β1,3-N-acetylglucosaminyltransferases (B3GNTs) are Golgi-resident glycosyltransferases involved in the biosynthesis of poly-N-acetyl-lactosamine chains. They catalyze the addition of the N-acetylglucosamine to the N-acetyl-lactosamine repeat as a key step of the chain elongation process. Among the characterized B3GNTs, B3GNT2 is the major poly-N-acetyl-lactosamine synthase, and deletion of its coding gene dramatically reduced the cell surface poly-N-acetyl-lactosamine and led to hypersensitive and hyperresponsive immunocytes. The luminal domain of B3GNT2 comprises an N-terminal helical domain (Pro55–Cys125) and a C-terminal catalytic domain (Cys138–Cys397) as well as an extended linker (Arg126–Lys137) that connects the helical domain to the catalytic domain.

By soaking B3GNT2 crystals with either the donor substrate UDP-GlcNAc or the acceptor substrate LacNAc, we were able to obtain B3GNT2 structures (B3GNT2_UDPGlcNAc and B3GNT2_LacNAc) in the substrate-bound states. In the B3GNT2_UDPGlcNAc structure, the donor substrate UDP-GlcNAc is positioned at the bottom of the cleft with the GlcNAc moiety close to the center of the cleft. The side chains of Asp215 and Lys223 are hydrogen bonded to the uracil ring of the UDP moiety, whereas the side chain of Asp246 is hydrogen bonded to the ribose hydroxyls. The pyrophosphate group of UDP clamps the divalent Mg ion in a bidentate manner. Two pyrophosphate oxygen atoms, Asp247 from the signature DXD motif (Asp245-Asp246-Asp247 in B3GNT2), a conserved His376, and two water molecules, coordinate the Mg ion with the tetragonal bipyramidal geometry. The side chains of Lys149, Asp245 (the other Asp from the signature DXD motif), Tyr289, and Asp332 are involved in hydrogen bond interactions with the GlcNAc moiety with Asp245 engaged in additional interaction with the nitrogen of the N-acetyl group. These interactions force the GlcNAc moiety to bend toward the cleft wall, almost perpendicular to the pyrophosphate and parallel to the uracil ring, and fully expose the C1 atom for the nucleophilic attack. And superposition of the B3GNT2_UDPGlcNAc and B3GNT2_LacNAc structures shows that the acceptor substrate LacNAc binds right above the donor substrate UDP-GlcNAc in the substrate-binding cleft. The hydroxyl group on C3 of the Gal in the acceptor substrate points to the C1 of the GlcNAc in the donor substrate at a distance of 3.7 Å. The Asp333, which is 2.7 Å from the hydroxyl group on C3 of Gal in the acceptor substrate LacNAc, serves as the active site base and abstracts the proton from this hydroxyl group. This facilitates the nucleophilic attack on the exposed C1 of the GlcNAc in the donor substrate UDP-GlcNAc, which undergoes an oxocarbenium ion–like transition state.

>[2x]MHHHHHHHHENLYFQGSKEKFWKISTPPEAYWNREQEKLNRQYNPILSMLTNQTGEAGRLSNISHLNYCEPDLRVTSVVTGFNNLPDRFKDFLLYLRCRNYSLLIDQPDKCAKKPFLLLAIKSLTPHFARRQAIRESWGQESNAGNQTVVRVFLLGQTPPEDNHPDLSDMLKFESEKHQDILMWNYRDTFFNLSLKEVLFLRWVSTSCPDTEFVFKGDDDVFVNTHHILNYLNSLSKTKAKDLFIGDVIHNAGPHRDKKLKYYIPEVVYSGLYPPYAGGGGFLYSGHLALRLYHITDQVHLYPIDDVYTGMCLQKLGLVPEKHKGFRTFDIEEKNKNNICSYVDLMLVHSRKPQEMIDIWSQLQSAHLKC> MSEPRFVHLRVHSDYSMIDGLAKTAPLVKKAAALGMPALAITDFTNLCGLVKFYGAGHGAGIKPIVGADFNVQCDLLGDELTHLTVLAANNTGYQNLTLLISKAYQRGYGAAGPIIDRDWLIELNEGLILLSGGRMGDVGRSLLRGNSALVDECVAFYEEHFPDRYFLELIRTGRPDEESYLHAAVELAEARGLPVVATNDVRFIDSSDFDAHEIRVAIHDGFTLDDPKRPRNYSPQQYMRSEEEMCELFADIPEALANTVEIAKRCNVTVRLGEYFLPQFPTGDMSTEDYLVKRAKEGLEERLAFLFPDEEERLKRRPEYDERLETELQVINQMGFPGYFLIVMEFIQWSKDNGVPVGPGRGSGAGSLVAYALKITDLDPLEFDLLFERFLNPERVSMPDFDVDFCMEKRDQVIEHVADMYGRDAVSQIITFGTMAAKAVIRDVGRVLGHPYGFVDRISKLIPPDPGMTLAKAFEAEPQLPEIYEADEEVKALIDMARKLEGVTRNAGKHAGGVVIAPTKITDFAPLYCDEEGKHPVTQFDKSDVEYAGLVKFDFLGLRTLTIINWALEMINKRRAKNGEPPL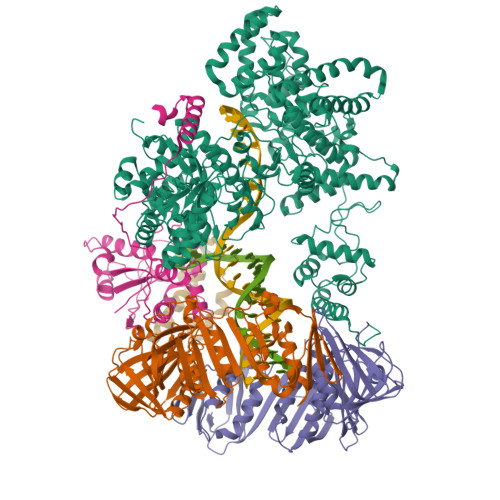DIAAIPLDDKKSFDMLQRSETTAVFQLESRGMKDLIKRLQPDCFEDMIALVALFRPGPLQSGMVDNFIDRKHGREEISYPDVQWQHESLKPVLEPTYGIILYQEQVMQIAQVLSGYTLGGADMLRRAMGKKKPEEMAKQRSVFAEGAEKNGINAELAMKIFDLVEKFAGYGFNKSHSAAYALVSYQTLWLKAHYPAEFMAAVMTADMDNTEKVVGLVDECWRMGLKILPPDINSGLYHFHVNDDGEIVYGIGAIKGVGEGPIEAIIEARNKGGYFRELFDLCARTDTKKLNRRVLEKLIMSGAFDRLGPHRAALMNSLGDALKAADQHAKAEAIGQLDLFGVL;>[2x]MKFTVEREHLLKPLQQVSGPLGGRPTLPILGNLLLQVADGTLSLTGTDLEMEMVARVALVQPHEPGATTVPARKFFDICRGLPEGAEIAVQLEGERMLVRSGRSRFSLSTLPAADFPNLDDWQSEVEFTLPQATMKRLIEATQFSMAHQDVRYYLNGMLFETEGEELRTVATDGHRLAVCSMPIGQSLPSHSVIVPRKGVIELMRMLDGGDNPLRVQIGSNNIRAHVGDFIFTSKLVDGRFPDYRRVLPKNPDKHLEAGCDLLKQAFARAAILSNEKFRGVRLYVSENQLKITANNPEQEEAEEILDVTYSGAEMEIGFNVSYVLDVLNALKCENVRMMLTDSVSSVQIEDAASQSAAYVVMPMRL;> MSTAITRQIVLDTETTGMNQIGAHYEGHKIIEIGAVEVVNRRLTGNNFHVYLKPDRLVDPEAFGVHGIADEFLLDKPTFAEVADEFMDYIRGAELVIHNAAFDIGFMDYEFSLLKRDIPKTNTFCKVTDSLAVARKMFPGKRNSLDALCARYEIDNSKRTLHGALLDAQILAEVYLAMTGGQLSLPLAMEGETQQQQGEATIQRIVRQASKLRVVFATDEEIAAHEARLDLVQKKGGSCLWRA;> QTEMDKVNVDLAAAGVAFKERYNMPVIAEAVEREQPEHLRSWFRERLIAHRLASVN>MKAVQYTEIGSEPVVVDIPTPTPGPGEILLKVTAAGLCHSDIFVMDMPAAQYAYGLPLTLGHEGVGTVAELGEGVTGFGVGDAVAVYGPWGCGACHACARGRENYCTRAADLGITPPGLGSPGS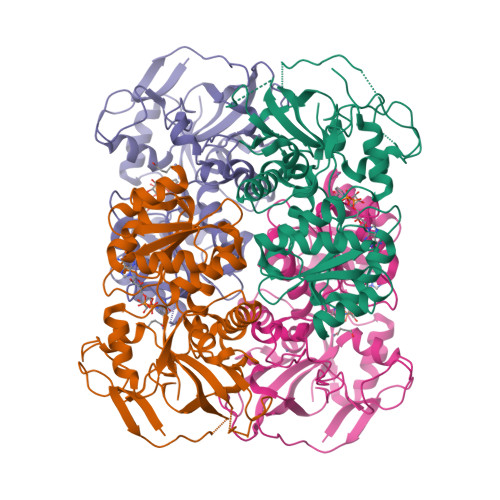MAEYMIVDSARHLVPIGDLDPVAAAPLTDAGLTPYHAISRVLPLLGPGSTAVVIGVGGLGHVGIQILRAVSAARVIAVDLDDDRLALAREVGADAAVKSGAGAADAIRELTGGQGATAVFDFVGAQSTIDTAQQVVAVDGHISVVGIHAGAHAKVGFFMIPFGASVVTPYWGTRSELMEVVALARAGRLDIHTETFTLDEGPAAYRRLREGSIRGRGVVVP[4x]> MQRSPVEDANCLSRYFFWWTNPIMRKGFKEKLRPSDVYQAPSQDAADILAERLEKEWDREVASGKKKPSLLRAMARCYIKPFLLFGFLLYIGEATKTVQPQLLGRIIASFDPAHEPERANGYFLAFGLGLLFTARFLLLQPAMFGLHHLGMQIRIALFSIIYKKTLKLSSRVLDKISTGQLVSLMSANLGKFDQSLGMAHFIWISPLQCILCTGLIWELIDVNSFCALAAISLLGVLQAFLSHKMGPYKAQKVLLTNKRLALTSEIMENLHSVKAYGWEEIMETLIKNIRQDEVKLTRKIGSLRYFYSSAYFFSAIFVIVAAVVPHALSRGINLRRIFTTLSYCMVLRMTVTRQLPGSIQMWYDTMRLIWKIEEFLSKEEYKLMEYDLSITELELQDVTASWDEGPGELLERIKQENKANGHHNGDAGLFFTNLYVAPVLKDISLKLKKGEMLAVTGSMGSGKSSLLMTILGELVPSSGKIRHSGRISYSSQTAWIMPGTIRDNILFGLTYDEYRYKSVVKACQLEEDLAALPEKDKTPMAEGGLNLSGGQKARVALARAVYRDADLYLLDAPFTHLDIATEKEIFDKCLCKLMASKTRILVTNKIEHLKRADKILLLHNGESFFYGTFPELQSERPDFSSLLLGLEAYDNISAERRCSILTETLHRVSVDESAGMQPERSAFRQVPPTKPMYIDERKASVIVNPLGVARKASFIQVPEEEVRRTLPDRKFSLVPENELVDESFMGSDVYHNHGVHMAGQRRQSVLAFMTNAQGQGRREHLQSSFRRRLSVVPQSELASELDIYTRRLSDSTYDMTGILEEENIEACLTDEIDEIEETFETTKWNTYVRYVSNNKSLLYVLIFILFIAAIEIAGSVAGIFLITDELWREEHQRSEPNMTKHSNASSSGQTYAITVTPTSSYYILYIYVATSESLLAMGFFRGLPFVHTTITISKKLHQKMLHAVLSAPMSVLNTMKTGRIMNRFTKDMA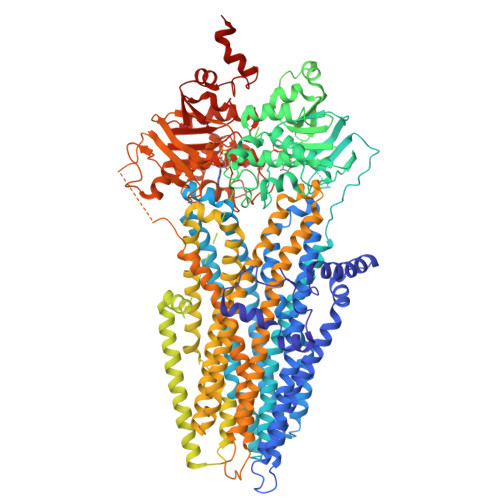TIDDMLPLLMFDFVQLTVVVVGCILVVSIVRPYIFLAATPLAIIFIVMRKYFLRTGQQLKQLETEARSPIFSHLIMSLKGLWTIRAFERQAYFEALFHKTLNTHTATWFLYLSTLRWFLFRADILFVFFFTLAAWIAVGTNQDKPGEIGIIICLAMLILGTFQWCVATSIAVDGMMRSVDRVFKFIDLPSETPKPDKGKDSDLIIENVDAQADSSWPHRGQIEVRNLTVKYTEAGHAVLKNLSFSAEGRQRVGILGRTGSGKSSLFNALLKLVYTDGEISIDGVNWNKMPLQKWRKAFGVVPQKVFIFTGPLRMNLDPYGCHSDEELWRVAEEVGLKTVIEQFPDKLDFQLEYGGYVLSNGHKQLICLARSILSGARILLLDQPSAHLDPVTIKVLKKTLRQSFSTCTILLSEHKVEPLLECQSFLMMDKGQVKTYDSIQKLLNETSHLKQAISPAERLKLFPRRNSSMRTPQSKLSSVTQTLQEEAEDNIQDTRLSNSLEVLFQ>[6x]A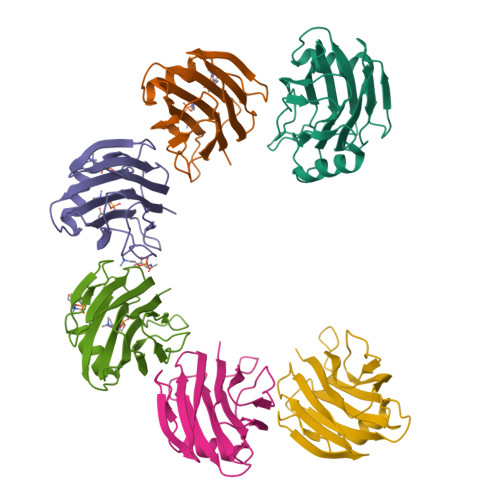LAGTIIAGASLTFQVLDKVLEELGKVSRKIAVGIDNESGGTWTALNAYFRSGTTDVILPEFVPNTKALLYSGRKDTGPVATGAVAAFAYYMSSGNTLGVMFSVPFDYNWYSNWWDVKIYSGKRRADQGMYEDLYYGNPYRGDNGWHEKNLGYGLRMKGIMTSAGEAKMQIKISR> MELKHSISDYTEAEFLQLVTTICNADTSSEEELVKLVTHFEEMTEHP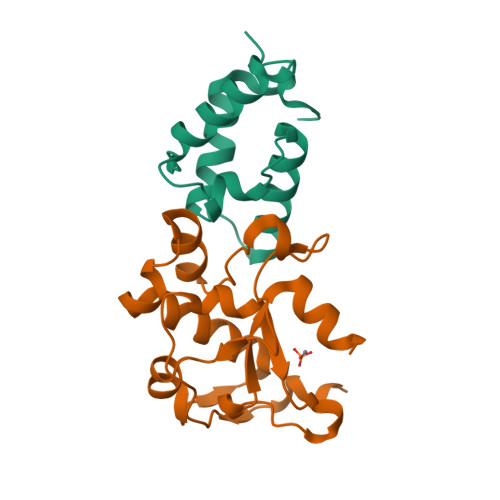SGSDLIYAPKEGDDDSPSGIVNTVKQWRAANGKSGFKQG;> MESKRNKPGKATGKGKPVGDKWLDDAGKDSGAPIPDRIADKLRDKEFKSFDDFRKAVWEEVSKDPELSKNLNPSNKSSVSKGYSPFTPKNQQVGGRKVYELHHDKPISQGGEVYDMDNIRVTTPKRHIDIHRGK> SMIPEVQKPLHEQLWYHGAIPRAEVAELLVHSGDFLVRESQGKQEYVLSVLWDGLPRHFIIQSLDNLYRLEGEGFPSIPLLIDHLLSTQQPLTKKSGVVLHRAVPKDKWVLNHEDLVLGEQIGRGNFGEVFSGRLRADNTLVAVKSCRETLPPDLKAKFLQEARILKQYSHPNIVRLIGVCTQKQPIYIVMELVQGGDFLTFLRTEGARLRVKTLLQMVGDAAAGMEYLESKCCIHRDLAARNCLVTEKNVLKISDFGMSREEADGVYAASGGLRQVPVKWTAPEALNYGRYSSESDVWSFGILLWETFSLGASPYPNLSNQQTREFVEKGGRLPCPELCPDAVFRLMEQCWAYEPGQRPSFSTIYQELQSIRKRHR;> XIYESL

We have solved the structure of the prototypic SH2-kinase unit of the human Fes tyrosine kinase, which appears specialized for positive signaling. We investigated the structure of a polypeptide from human Fes comprising a linker region N terminal to the SH2 domain, the SH2 domain, and the C-terminal kinase domain. The three structures were determined in complex with the ATP mimetic kinase inhibitor staurosporine and were refined to low R factors and acceptable geometry. The SH2 domain, the kinase domain, and substrate apparently interact cooperatively to yield a functional Fes kinase complex.

To better understand Fes regulation, we also solved structures of unphosphorylated Fes in the absence of phosphomimetic salt ions and Fes in which the regulatory activation segment residue (Y713) had been autophosphorylated in vitro. In both cases, a substrate peptide (IYESL) was cocrystallized. As expected, in phosphorylated Fes, the phosphorylated Y713 formed a network of salt bridges and hydrogen bonds of the sort typically observed in activation segments of activated kinases. This links the conserved catalytic loop arginine (R682) with the activation segment and additionally stabilizes the active conformation through hydrogen bonds to R706 and S716. Second, binding of the substrate peptide also induces a β sheet secondary structure between the substrate peptide and a strand in the activation segment (βI), with typical main chain hydrogen bond interactions. Selectivity for hydrophobic interactions in substrate positions −1 and +3 can be explained by binding of the corresponding substrate residues isoleucine and leucine to hydrophobic pockets on the Fes kinase, and selectivity for acidic residues in position +1 is due to formation of a hydrogen bond with N766 located in helix αG. The binding mode of staurosporine to the ATP pocket is similar to structures reported previously (Bertrand et al., 2003); in addition, two molecules of staurosporine were identified in crystal contacts in Fes-substrate complexes. A striking feature of both structures was the large degree of disorder in SH2 domain loop regions as well as in the loop connecting the sheet β3 with αC. In addition, helix αC showed very high temperature factors, indicating a high degree of mobility of this regulatory element.>MRGG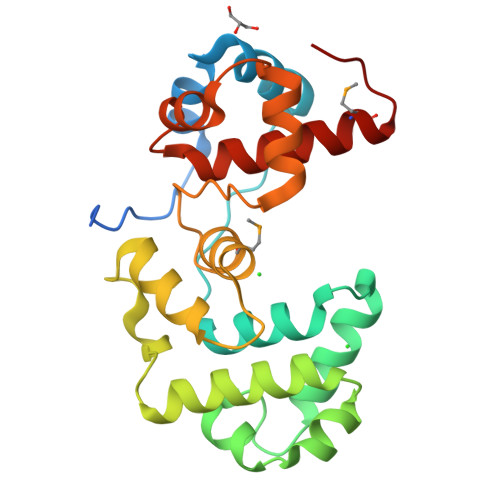ALHQNRRVTLPSVPLPAVLPPLTDHAGAVAHLSRDPVLAQVTSLCGELPVLAPTPDPFGRLVRSVAGQQLSVKAAQAIYGRLEGLPGGVVPAALLKVSGDDLRGVGLSWAKVRTVQAAAAAAVSGQIDFAHLSGQPDELVIAELVQLPGIGRWTAEMFLLFALARPDVFSSGDLALRQGVERLYPGEDWRDVTARWAPYRSLASRYLWANSARMQAGGAPL[2x]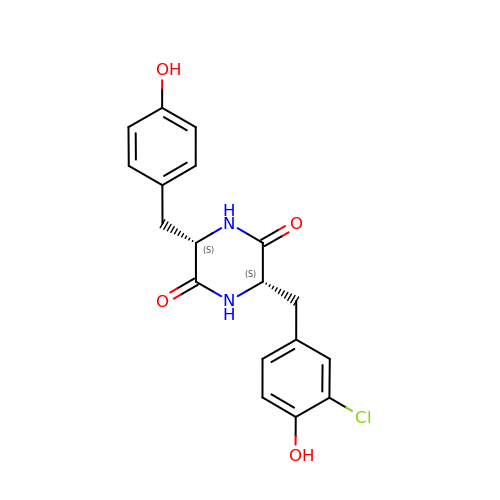(3~{S},6~{S})-3-[(3-chloranyl-4-oxidanyl-phenyl)methyl]-6-[(4-hydroxyphenyl)methyl]piperazine-2,5-dione | C18 H17 Cl N2 O4 | DPXFBAHRLYLKSZ-GJZGRUSLSA-N>PCKFYICSNWEAIHKSCPGNT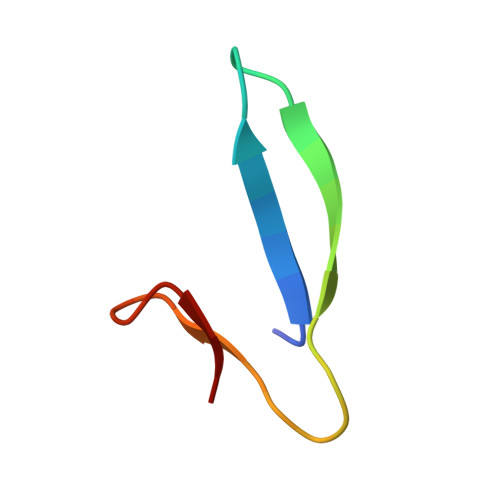RWNEKELTCT[2x]> MAAQLSEQLAELEKRSGGRLGVAVLDTATGRRIAYRGDERFPMCSTFKALLAAAVLARVDQGKERLDRRITYGKEDLVDYSPVTEKHVGDGMTVAELCEAAITLSDNTAANLLLEALGGPAALTAFLRSIGDEVTRLDRWEPELNEAAPGDPRDTTTPAAMAATLRTLLLGDALSPASRQQLVDWLVANKTGDKRLRAGLPADWRVGDKTGTGGHGTTNDIAVIWPPGRAPIVVTVYLTESQVDADARDAVIAEVGRLVVEAFHHHHHH

Here, we explore and test these notions using resurrected Precambrian β-lactamases11 as scaffolds for the engineering of completely new active sites. Of these systems, resurrected Precambrian β-lactamases have been thoroughly characterized in terms of their structure, function and stability. These putative ancestral proteins have been shown to be highly stable and able to efficiently degrade several antibiotics. A hydrophobic-to-ionizable amino acid replacement generates a buried (or partially buried) residue with the perturbed properties that are useful in catalysis and conformational flexibility assists the generation of a completely new active site by facilitating substrate and transition-state binding. We have shown that, when using resurrected Precambrian β-lactamases as scaffolds for protein engineering, a minimalist design approach based on this mechanism leads to levels of catalysis for the Kemp elimination reaction of up to approximately seven orders of magnitude above the rate of the uncatalysed reaction, as well as to significant ester hydrolysis activity.

Consequently, we used NMR relaxation determinations (see Methods section and Supplementary Methods) on the β-lactamase encoded by the most probabilistic sequence at the GNCA node (GNCAMP β-lactamase) to guide our design of a new active site. This putative ancestral protein displays a large number of residues with conformational contribution to the relaxation rates determined by NMR (see the comparison with the modern TEM-1 β-lactamase shown in Fig. 3). A large accumulation of such residues is visually apparent in the region encompassing helix h1 (residues 26–41), helix h11 (residues 271–290) and the loops 225–229 and 252–257. Residue 229 within this region appears as a suitable target for the generation of a new active site through a hydrophobic-to-ionizable residue replacement. A substantially buried and highly conserved tryptophan residue is present at position 229 in both modern and reconstructed Precambrian β-lactamases. In the case of the wild-type enzymes, a clear increase can be seen in the flexibility of residues 252 through to the h11 helix upon moving from TEM-1 and BL to the GNCAMP to GNCA4 β-lactamases, which are the residues that are primarily involved in forming the cavity creating the de novo active site. The flexibility of this region appears indeed to follow the general activity trend described above.>MAPKQTPSPEKNRNLVGPVLQRRQTEGTFDQRLLEMRADHNWKHADPWRVLRI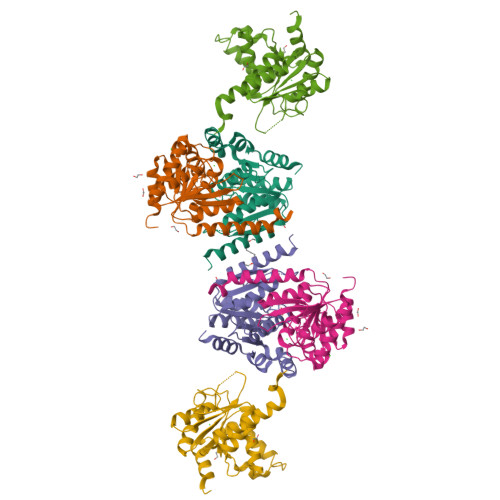QSEFVAGFDALHEMPKAVTVFGSARIKEDHPYYKAGVELGEKLVAADYAVVTGGGPGLMEAPNKGASEANGLSVGLGIELPHEQHLNPYVDLGLNFRYFFARKTMFLKYSQAFVCLPGGFGTLDELFEVLCMVQTGKVTNFPIVLIGTEFWAGLVDWIRHRLVEEGMIDEKDVDRMLVTDDLDQAVKFIVDAHAGLDVARRHNLEHHHHHH[3x]>MSSAIKEVQGAPVKWVTNWTPEAIRGLVDQEKGLLDPRIYADQSLYELELERVFGRSWLLLGHESHVPETGDFLATYMGEDPVVMVRQKDKSIKVFLNQCRHRGMRICRSDAGNAKAFTCSYHGWAYDIAGKLVNVPFEKEAFCDKKEGDCGFDKAEWGPLQARVATYKGLVFANWDVQAPDLETYLGDARPYMDVMLDRTPAGTVAIGGMQKWVIPCNWKFAAEQFCSDMYHAGTTTHLSGILAGIPPEMDLSQAQIPTKGNQFRAAWGGHGSGWYVDEPGSLLAVMGPKVTQYWTEGPAAELAEQRLGHTGMPVRRMVGQHMTIFPTCSFLPAMNNIRIWHPRGPNEIEVWAFTLVDADAPAE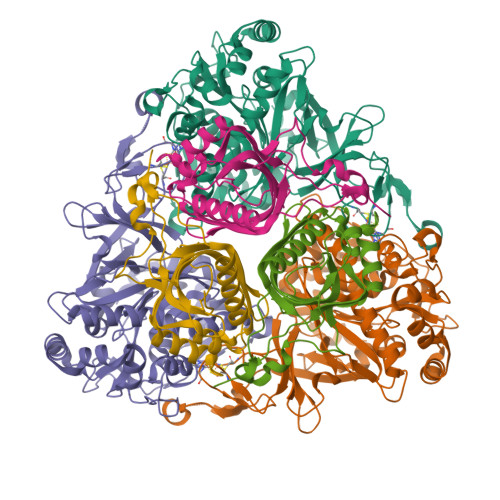IKEEYRRHNIRNFSAGGVFEQDDGENWVEIQKGLRGYKAKSQPLNAQMGLGRSQTGHPDFPGNVGYVYAEEAARGMYHHWMRMMSEPSWATLKP[12x];>[12x]MTNPSPHFFKTFEWPSKAAGLELQNEIEQFYYREAQLLDHRAYEAWFALLDKDIHYFMPLRTNRMIREGELEYSGDQDLAHFDETHETMYGRIRKVTSDVGWAENPPSRTRHLVSNVIVKETATPDTFEVNSAFILYRNRLERQVDIFAGERRDVLRRADNNLGFSIAKRTILLDASTLLSNNLSMFF> ANPRYKIPVEADFLFAYSTVPGYYSWRSPGRGSWFVQALCSILEEHGKDLEIMQILT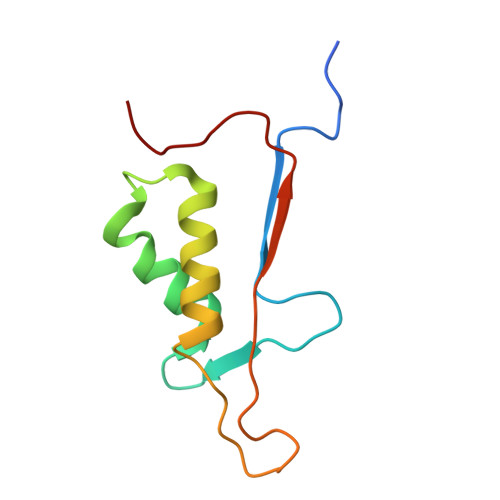RVNDRVARHFESQSDDPHFHEKKQIPCVVSMLTKELYFSQ>MGADDVVDSSKSFVMENFSSYHGTKPGYVDSIQKGIQKPKSGTQGNYDDDWEGFYSTDNKYDAAGYSVDNENPLSGKAGGVVKVTYPGLTKVLALKVDNAETIKKELGLSLTEPLMEQVGTEEFIKRFGDGASRVVLSLPFAEGSSSVKYINNWEQAKALSVELEINFETRGKRGQDAMYEYMAQACAGNRVRRSVGSSLSCINLDWDVIRDKTKTKIESLKEHGPIKNKMSESPNKTVSEEKAKQYLEEFHQTALEHPELSELKTVTGTNPVFAGANYAAWAVNVAQVIDSETADNLEKTTAALSILPGIGSVMGIADGAVHHNTEEIVAQSIALSSLMVAQAIPLVGELVDIGFAAYNFVESIINLFQVVHNSYNRPAYSPGHKTQPFLHDGYAVSWNTVEDSIIRTGFQGESGHDIKITAENTPLPIAGVLLPTIPGKLDVNKSKTHISVNGRKIRMRCRAIDGDVTFCRPKSPVYVGNGVHANLHVAFHRSSSEKIHSNEISSDSIGVLGYQKTVDHTKVNSKLSLFFEIKSMA[2x]

Diphtheria toxin (DT) is secreted by Corynebacterium and causes disease in humans by inhibiting protein synthesis. DT consists of three domains—receptor (R-), translocation (T-), and catalytic (C-)—and similar to many other A-B toxins it enters the cell via the endosomal pathway. After the binding of the R-domain to the EGFR-like receptor on the cell surface, the toxin is endocytosed into the cell, and acidification inside the endosome promotes the requisite conformational change and membrane insertion of the T-domain followed by the translocation of the C-domain into the cytosol. Following translocation, the C-domain is proteolyzed from the R and T domains and proceeds to inhibit the EF2 translation factor, leading to the termination of protein synthesis and cell death.

DT was crystallized under varying buffer conditions in an effort to determine if conformational changes, particularly in the T-domain, are observed with a decreasing pH. Since the crystallization conditions were identical except for the buffer, the crystals of DT-5.0, DT-5.5, DT-6.0, and DT-7.0 have similar unit cell dimensions and diffraction resolutions. However, the α-angle for DT-5.0 is approximately 4° larger than that of other crystals. The structures of DT at various pH values were superimposed onto DT-5.0 using GESAMT in order to compare their similarities/differences. Overall, all of the structures are very similar, with RMSD deviations between the Cα atoms of 0.34 Å (997 residues, DT-5.5), 0.38 Å (999 residues, DT-6.0), and 0.41 Å (1000 residues, DT-7.0). Interestingly, the residues between H223 to P234, which span TH2, appear to become more flexible at a lower pH. In the DT-5.0 structure, the TH2 helix could be modelled in subunit A but not subunit B. It should be noted that this region does not form any crystal contacts that would cause conformational artifacts. In contrast, the long TH1, which is also expected to refold based on the latter studies, remains unchanged in the crystal structure even at pH 5. Surprisingly, the TH1 helix maintains its conformation in the crystal of the full-length toxin even at pH 5. We demonstrate that neither catalytic nor receptor-binding domains change their structure upon this acidification, while the T-domain undergoes a conformational change that results in the unfolding of TH2–3 helices.>SMTTLFSKIKEVTELAAVSGHEAPVRAYLREKLTPHVDEVVTDGLGGIFGIKHSEAVDAPRVLVASHMDEVGFMVSEIKPDGTFRVVEIGGWNPMVVSSQRFKLLTRDG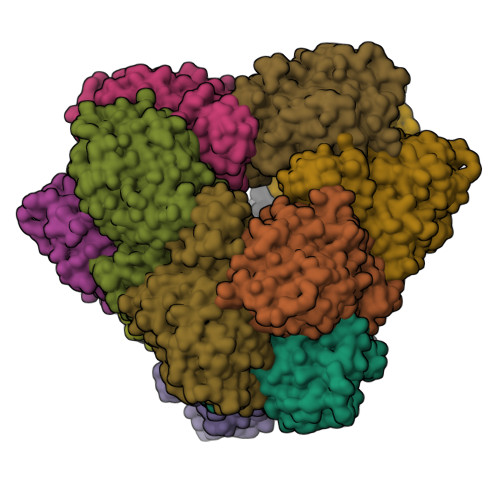HEIPVISGSVPPHLTRGKGGPTMPAIADIVFDGGFADKAEAESFGIRPGDTIVPDSSAILTANEKNIISKAWDNRYGVLMVSELAEALSGQKLGNELYLGSNVQEEVGLRGAHTSTTKFDPEVFLAVDCSPAGDVYGGQGKIGDGTLIRFYDPGHLLLPGMKDFLLTTAEEAGIKYQYYCGKGGTDAGAAHLKNGGVPSTTIGVCARYIHSHQTLYAMDDFLEAQAFLQALVKKLDRSTVDLIKHY[12x]>MSQTLLVHGKDAQGIIKQVLSEVYDAVTSTMGPNGQLVMIKNGVSTKTTKDGVTVARSIRFADEAHELVNRVITEPATKTDEECGDGTTTTIMLTHALYHLFKDFPGFQHHRNIEDLVERVIQRLESMAIRVEVDDPRLYQVALTSSNQDEKLARLVSELYANNKGSYPDIELKEGVNFEDQIEQTTGRTIRMFYANPWFAKGHQGGVTELTGFTAFVIDRRIDKEDTQKLIDGVNHLVKTHKQHLALPILLIARSFEEAANSTLMQLNAAHPTLVEDGRPWLIPLSTPVGGAIGTSELQDIAVMLNAPMLSDVADLTKLDTHSINGQHGQLELGGNRSILKSTTPKDEDRIEQHARGIEELLEGFSLSDKFSVRARYNERRIRTLRGKLITISVGGETYSEVKERVDRYEDVVKAIRSALENGILPGGGVSLVKAVFGTIKEGLEDKDQSAEFAKRYINSGIANELMRLSTIQHKLLFKDTALYKENGSFHFNDDWLNTPTVMNLATGEIGTPEGLGIYDTAYASITALKGGLQTAKILATTKTLILGEKLSAVKVR[7x]

Our structural and functional analysis of the chaperonin ɸEL from the bacteriophage EL of P. aeruginosa revealed that the protein is ATPase active and functions in aggregation prevention of denatured proteins. ɸEL forms tetradecameric double ring complexes, which dissociate into a population of single rings in the presence of ATP and at physiological salt concentration. As anticipated, the ɸEL subunits displayed the typical three-domain architecture of chaperonins, composed of an equatorial domain (residues 2–130 and 425–552), an intermediate domain (residues 131–188 and 388–424), and an apical domain (residues 189–387). The domain structures of ɸEL differ from those of GroEL by numerous insertions and deletions, which alter the putative substrate-binding cleft and the contacts at the ring-ring interface. Our functional data rather suggests that the chaperone mechanism of ɸEL is encapsulation independent, and represents an evolutionary precursor of the more complex encapsulation mechanisms used by the group I and II chaperonins.

The ɸEL heptamer in crystal form I (4.03 Å resolution) consisted of subunits in closely similar conformations (conformation I, r.m.s.d. range for Cα positions 0.28–1.36 Å). In conformation I, the tip of the protruding αK-αL helical hairpin of the apical domain contacts the equatorial domain. The αK-αL helical hairpin makes additional contacts to the intermediate domain. These contacts appear to stabilize the orientation of the apical domain. All subunits as judged from the electron density had either ATP or ADP•BeFX bound in the equatorial domain. For simplicity, we modelled the bound nucleotide as ATP. ATP was cradled by the αA-β2 loop (residues 30–33), the N-terminal ends of helix αD (residues 86–90) and helix αN1 (residues 428–430), helix αO (residues 474 and 478) and residues 504–506 and 519–521. Intermediate domain helix αM with the catalytic residue Asp412 (equivalent to Asp398 in E. coli GroEL) was at ~6.5 Å distance to the γ-phosphate of ATP, consistent with a conformation poised for ATP hydrolysis. In crystal form I, the putative SP binding site is solvent exposed, consistent with the ability of ɸEL to bind SP in the presence of ATP. The other crystal form was solved by molecular replacement using this model. Both structures consist of heptameric single-ring complexes of ɸEL.3-[4-(morpholin-4-yl)-7H-pyrrolo[2,3-d]pyrimidin-5-yl]benzonitrile 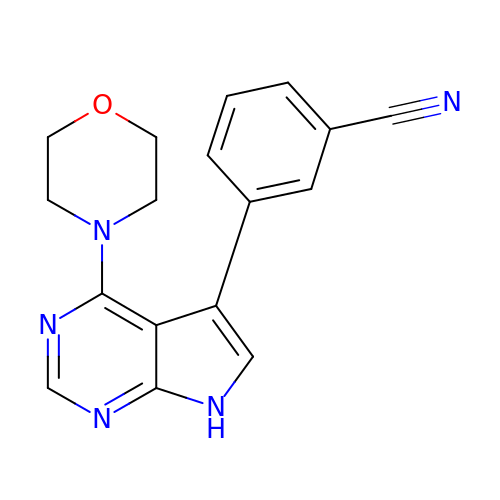| C17 H15 N5 O | BHTWDJBVZQBRKP-UHFFFAOYSA-N>[6x]MSASQKEGKLSTATISVDGKSAEMPVLSGTLGPDVIDIRKLPAQLGVFTFDPGYGETAACNSKITFIDGDKGVLLHRGYPIAQLAENASYEEVIYLLLNGELPNKAQYDTFTNTLTNHTLLHEQIRNFFNGFRRDAHPMAILCGTVGALSAFYPDANDIAIPANRDLAAMRLIAKIPTIAAWAYKYTQGEAFIYPRNDLNYAENFL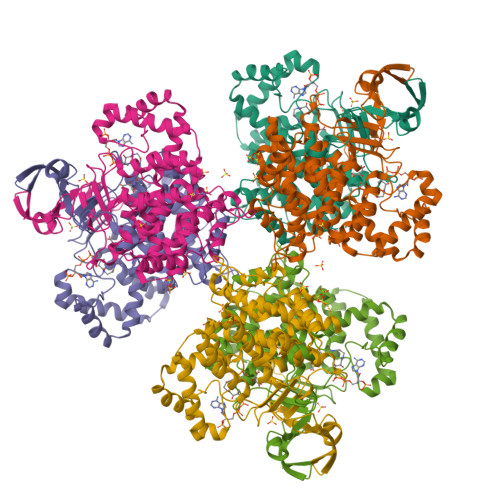SMMFARMSEPYKVNPVLARAMNRILILHADHEQNASTSTVRLAGSTGANPFACIAAGIAALWGPAHGGANEAVLKMLARIGKKENIPAFIAQVKDKNSGVKLMGFGHRVYKNFDPRAKIMQQTCHEVLTELGIKDDPLLDLAVELEKIALSDDYFVQRKLYPNVDFYSGIILKAMGIPTSMFTVLFAVARTTGWVSQWKEMIEEPGQRISRPRQLYIGAPQRDYVPLAKR>NLYFQSMMLDRIRVVLVNTSHPGNIGGAARAMKNMGLSQLVLVQPESFPHGDAVARAS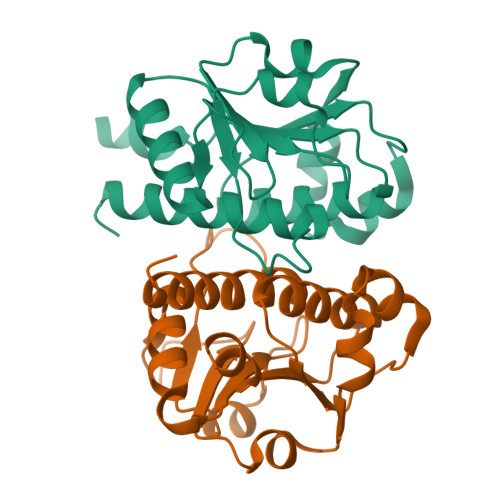GATDILDAARVVDTLEEALSGCSVVLGTSARDRRIPWPLLDPRECATTCLEHLEANGEVALVFGREYAGLTNEELQRCQFHVHIPSDPEFGSLNLAAAVQVLTYEVRMAWLAAQGK[4x]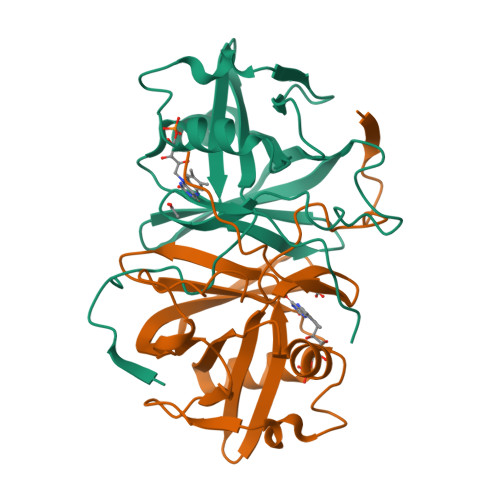>[2x]MRSYRAQGPLPGFYHYYPGVPAVVGVRVEERVNFCPAVWNTGLSADPPLFGVSISPKRFTHGLLLKARRFSASFHPFGQKDLVHWLGSHSGREVDKGQAPHFLGHTGVPILEGAYAAYELELLEVHTFGDHDLFVGRVVAVWEEEGLLDEKGRPKPGLALLYYGKGLYGRPAEETFAP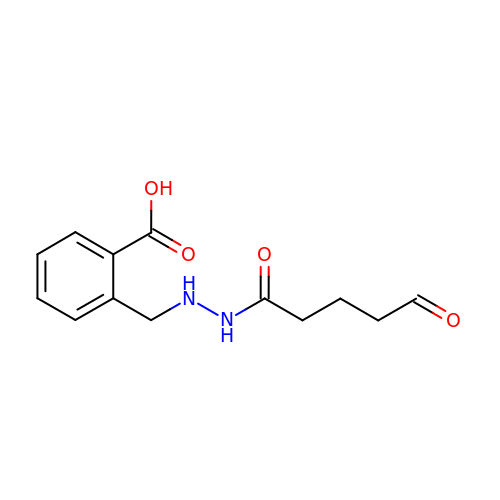2-[[2-(5-oxidanylidenepentanoyl)hydrazinyl]methyl]benzoic acid | C13 H16 N2 O4 | WAEOIFKXEDZIQC-UHFFFAOYSA-N> MSWRILLCHKHPVSARLRFLIPTGGGVVLPQTLPRLAVIAEDQEAPVQCHPASALRALQETMALGWQLELIGEFRLNMEVPGQIMPIYLAALAGHELPP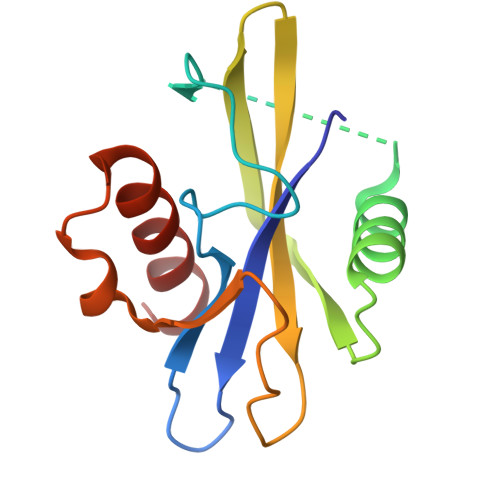PPEGTRWIELTQSIGMPWLDRELLRRVYEELIG> HQLYIDETVNSNIPTNLRVLRSILENLRSKIQKLESDVSAQMEYCRTPCTVSCNIPVVSGKECEEIIRKGGETSEMYLIQPDSSVKPYRVYCDMNTENGGWTVIQNRQDGSVDFGRKWDPYKQGFGNVATNTDGKNYCGLPGEYWLGNDKISQLTRMGPTELLIEME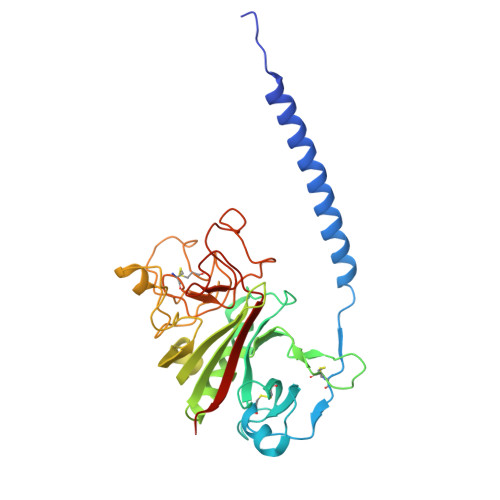DWKGDKVKAHYGGFTVQNEANKYQISVNKYRGTAGNALMDGASQLMGENRTMTIHNGMFFSTYDRDNDGWLTSDPRKQCSKEDGGGWWYNRCHAANPNGRYYWGGQYTWDMAKHGTDDGVVWMNWKGSWYSMRKMSMKIRPFFPQQ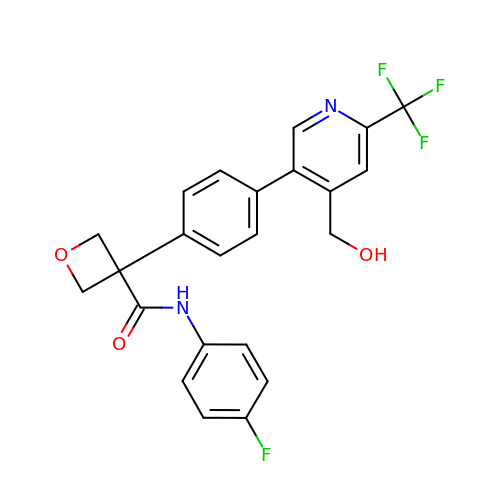N-(4-fluorophenyl)-3-{4-[4-(hydroxymethyl)-6-(trifluoromethyl)pyridin-3-yl]phenyl}oxetane-3-carboxamide | C23 H18 F4 N2 O3 | KTZHBUHZJXHRMG-UHFFFAOYSA-N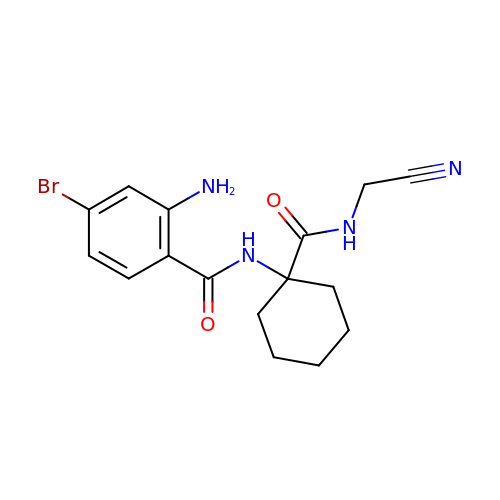2-amino-4-bromo-N-{1-[(cyanomethyl)carbamoyl]cyclohexyl}benzamide | C16 H19 Br N4 O2 | KVQZUZVIKTWMTQ-UHFFFAOYSA-N>[2x]MESEGKIVFTEEQEALVVKSWSVM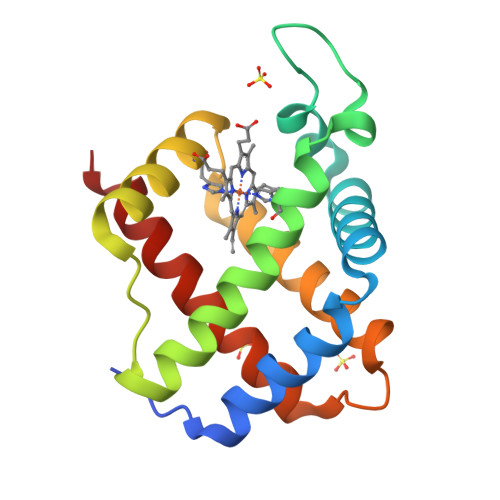KKNSAELGLKLFIKIFEIAPTTKKMFSFLRDSPIPAEQNPKLKPHAMSVFVMCCESAVQLRKTGKVTVRETTLKRLGASHSKYGVVDEHFEVAKYALLETIKEAVPEMWSPEMKVAWGQAYDHLVAAIKAEMNLSN>ASPKRSDGTPFPWNKIRLPEYVIPVHYDLLIHANLTTLTFWGTTKVEITASQPTSTIILHSHHLQISRATLRKGAGERLSEEPLQVLEHPRQEQIALLAPEPLLVGLPYTVVIHYAGNLSETFHGFYKSTYRTKEGELRILASTQFEPTAARMAFPCFDEPAFKASFSIKIRREPRHLAISNMPLVKSVTVAEGLIEDHFDVTVKMSTYLVAFIISDFESVSKITKSGVKVSVYAVPDKINQADYALDAAVTLLEFYEDYFSIPYPLPKQDLAAIPDFQSGAMENWGLTTYRESALLFDAEKSSASSKLDITMTVAHELAHQWFGNLVTMEWWNDLWLNEGFAKFMEFVSVSVTHPELKVGDYFFGKCFDAMEVDALNSSHPVSTPVENPAQIREMFDDVSYDKGACILNMLREYLSADAFKSGIVQYLQKHSYKNTKNEDLWDSMASICPTDGVKGMDGFCSRSQHSSSSSHWHQERVDVKTMMNTWTLQRGFPLITITVRGRNVHMKQEHYMKGSDGAPDTGYLWHVPLTFITSKSDMVHRFLLKTKTDVLILPEEVEWIKFNVGMNGYYIVHYEDDGWDSLTGLLKGTHTAVSSNDRASLINNAFQLVSIGKLSIEKALDLSLYLKHETEIMPVFQGLNELIPMYKLMEKRDMNEVE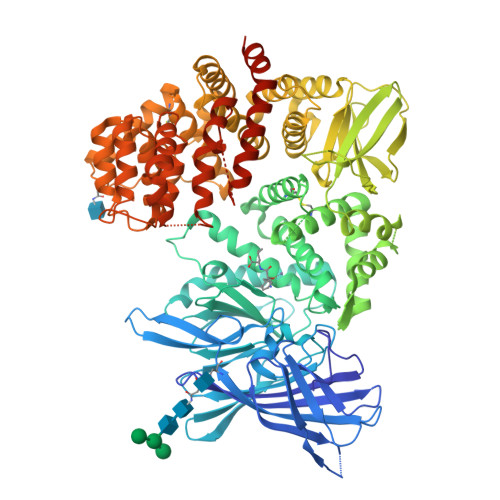TQFKAFLIRLLRDLIDKQTWTDEGSVSERMLRSELLLLACVHNYQPCVQRAEGYFRKWKESNGNLSLPVDVTLAVFAVGAQSTEGWDFLYSKYQFSLSSTEKSQIEFALCRTQNKEKLQWLLDESFKGDKIKTQEFPQILTLIGRNPVGYPLAWQFLRKNWNKLVQKFELGSSSIAHMVMGTTNQFSTRTRLEEVKGFFSSLKENGSQLRCVQQTIETIEENIGWMDKNFDKIRVWLQSEKLEHDPEADATGLERMLESRG[3x]>[2x]MSKSSMSTPNIAFPAITQEQMSSIKVDPTSNLLPSQEQLKSVSTLMVAAKVPAASVTTVALELVNFCYDNGSSAYTTVTGPSS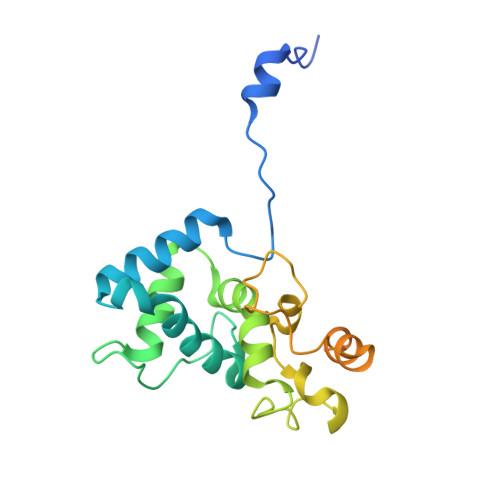IPEISLAQLASIVKASGTSLRKFCRYFAPIIWNLRTDKMAPANWEASGYKPSAKFAAFDFFDGVENPAAMQPPSGLTRSPTQEERIANATNKQVHLFQAAAQDNNFASNSAFITKGQISGSTPTIQFLPPPETSTTRHHHHHH> MAHHHHHHSAALEVLFQGPGNNELSPVALRQMSCAAGTTQTACTDDNALAYYN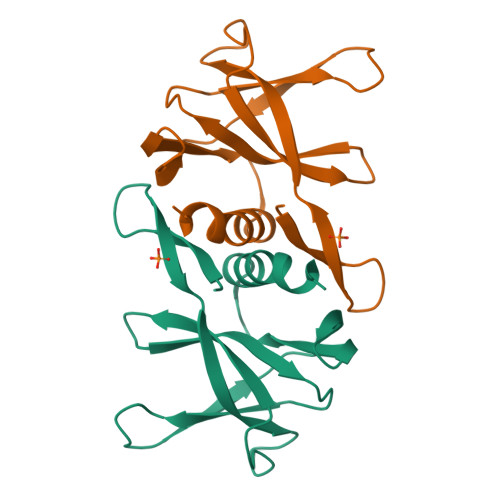TTKGGRFVLALLSDLQDLKWARFPKSDGTGTIYTELEPPCRFVTDTPKGPKVKYLYFIKGLNNLNRGMVLGSLAATVRLQ>[2x]PGAPWWKSAVFYQVYPRSFKDTNGDGIGDFKGLTEKLDYLKGLGIDAIWINPHYASPNTDNGYDISDYREVMKEYGTMEDFDRLMAELKKRGMRLMVDVVINHSSDQHEWFKSSRASKDNPYRDYYFWRDGKDGHEPNNYPSFFGGSAWEKDPVTGQYYLHYFGRQQPDLNWDTPKLREELYAMLRFWLDKGVSGMRFDTVATYSKTPGFPDLTPEQMKNFAEAYTQGPNLHRYLQEMHEKVFDHYDAVTAGEIFGAPLNQVPLFIDSRRKELDMAFTFDLIRYDRALDRWHTIPRTLADFRQTIDKVDAIAGE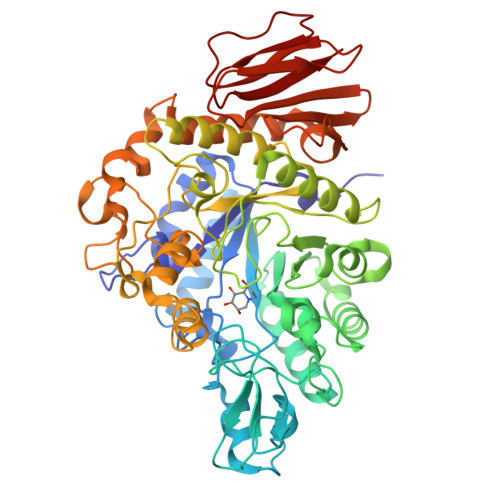YGWNTFFLGNHDNPRAVSHFGDDRPQWREASAKALATVTLTQRGTPFIFQGDELGMTNYPFKTLQDFDDIEVKGFFQDYVETGKATAEELLTNVALTSRDNARTPFQWDDSANAGFTTGKPWLKVNPNYTEINAAREIGDPKSVYSFYRNLISIRHETPALSTGSYRDIDPSNADVYAYTRSQDGETYLVVVNFKAEPRSFTLPDGMHIAETLIESSSPAAPAAGAASLELQPWQSGIYKVK>[4x]RKCSLTGKWTNDLGSNMTIGAVNSRGEFTGTYITAVT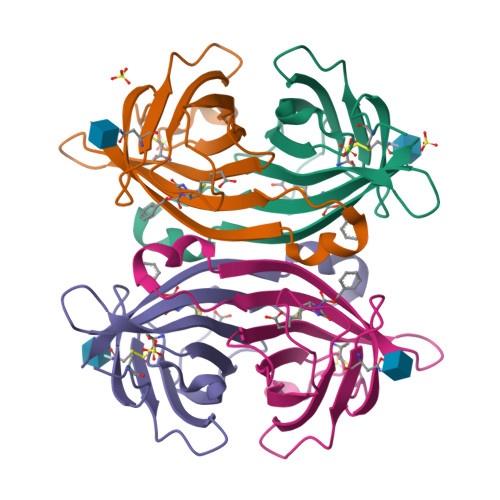ATSNEIKESPLHGTQNTINKRTQPTFGFTVNWKFSESTTVFTGQCFIDRNGKEVLKTMWLLRSSVNDIGDDWKATRVGINIFTRL> GSMAGNFWQSSHYLQWILDKQDLLKERQK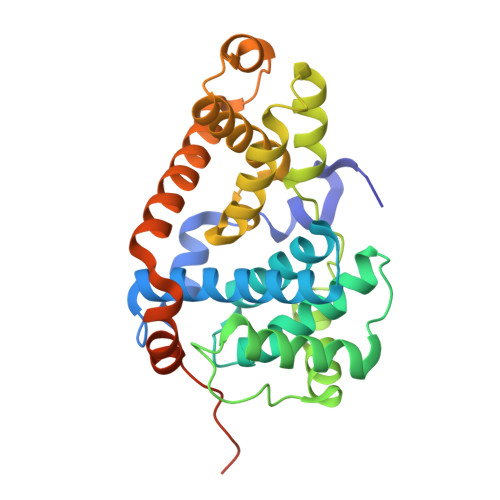DLKFLSEEEYWKLQIFFTNVIQALGEHLKLRQQVIATATVYFKRFYARYSLKSIDPVLMAPTCVFLASKVEEFGVVSNTRLIAAATSVLKTRFSYAFPKEFPYRMNHILECEFYLLELMDCCLIVYHPYRPLLQYVQDMGQEDMLLPLAWRIVNDTYRTDLCLLYPPFMIALACLHVACVVQQKDARQWFAELSVDMEKILEIIRVILKLYEQWKNFDERKEMATILSKMPKPKPPPNSEGEQGPNGSQNSSYSQS>GSFTEELHLIPPLNFSMVDNGIFRSGFPDSANFSFLQTLGLRSIIYLCPEPYPESNLQFLKSNGIRLFQFGIEGNKEPFVNIPDHKIRMALKVLLDEKNHPVLIHCKRGKHRTGCLVGCLRKLQKWCLTSIFDEYQRFAAAKARVSDQRFMEIFDVSSFSHIPMSFSCSI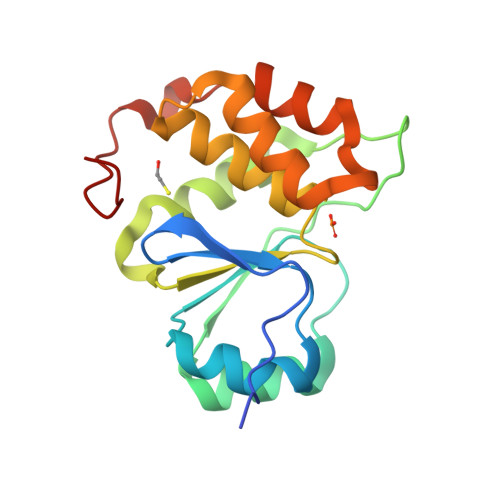R[2x]>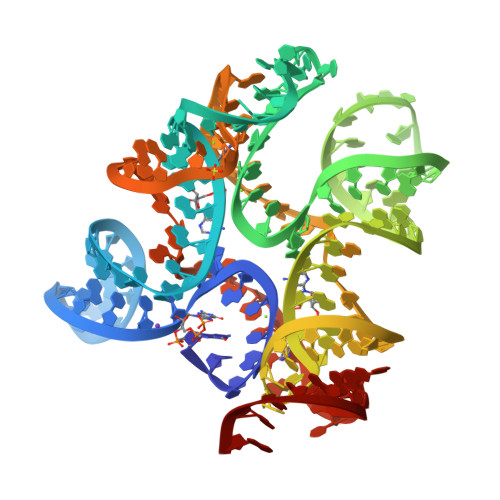 GGUUGCCGAAUCCACCUAGAAAUGGUACGGAGGAACCGCUUUUUGGGGUUAAUCUGCAGUGAAGCUGCAGUAGGGAUACCUUCUGUCCCGCACCCGACAGCUAACUCCGGAGGCAAUAAAGGAAGGAG N-{4-chloro-3-[4-(trifluoromethyl)-1,3-thiazol-2-yl]phenyl}-N'-(2-{3-[(1E)-N-hydroxyethanimidoyl]phenyl}propan-2-yl)urea 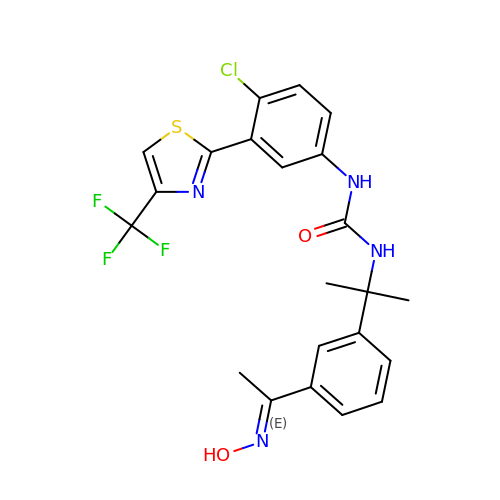| C22 H20 Cl F3 N4 O2 S | RTMPYAODZXTXJR-PNQUVVCRSA-N>[4x]MQKPVCLVVAMTPKRGIGINNGLPWPHLTTDFKHFSRVTKTTPEEASRLNGWLPRKFAKTGDSGLPSPSVGKRFNAVVMGRKTWESMPRKFRPLVDRLNIVVSSSLKEEDIAAEKPQAEGQQRVRVCASLPAALSLLEEEYKDSVDQIFVVGGAGLYEAALSLGVASHLYITRVAREFPCDVFFPAFPGDDILSNKSTAAQAAAPAESVFVPFCPELGREKDNEATYRPIFISKTFSDNGVPYDFVVLEKRRKTDDAATAEPSNAMSSLTSTRETTPVHGLQAPSSAAAIAPVLAWMDEEDRKKREQKELIRAVPHVHFRGHEEFQYLDLIADIINNGRTMDDRTGVGVISKFGCTMRYSLDQAFPLLTTKRVFWKGVLEELLWFIRGDTNANHLSEKGVKIWDKNVTREFLDSR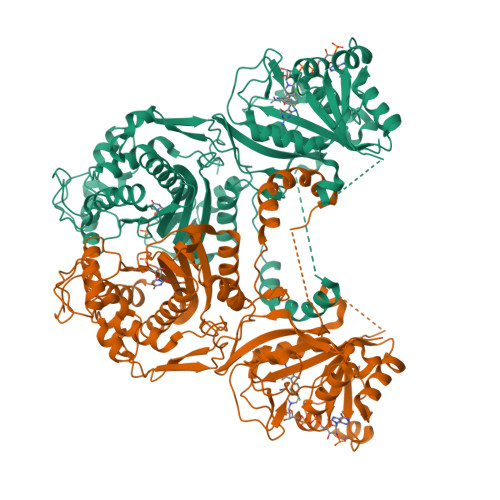NLPHREVGDIGPGYGFQWRHFGAAYKDMHTDYTGQGVDQLKNVIQMLRTNPTDRRMLMTAWNPAALDEMALPPCHLLCQFYVNDQKELSCIMYQRSCDVGLGVPFNIASYSLLTLMVAHVCNLKPKEFIHFMGNTHVYTNHVEALKEQLRREPRPFPIVNILNKERIKEIDDFTAEDFEVVGYVPHGRIQMEMAV> ATYMLPSLHDILDQHTYKWIFFGGKGGVGKTTTSSSFSVLMAETRPNEKFLLLSTNPAHNISDAFDQKFGKAPTQVSGIPNLYAMEVDASNEMKSAVEAVQKETGSAADNDAESKSEGDMFGGLNDLITCASSFIKDGTFPGMDEMWSFINLIKLIDTNEYSTVIFDTAPTGHTLRFLELPETVNKVLEIFTRLKDNMGGMLSMVMQTMGLSQNDIFGLIDKTYPKIDVVKRISAEFRDPSLCTFVGVCIPEFLSLYETERLVQRLAV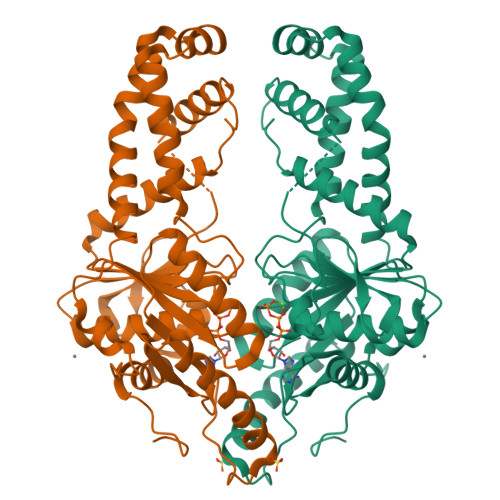LDMDCHAIVINFVLDANAATPCSMCRSRARMQNKYIDQINELYDDFNIVLSPLRHDEVRGIANLRDYAETLIKPYRFCWSANPDPSSAK> RSLLKTKENLGSGFISLFRGKKIDDDLFEELEEQLLIADVGVETTRKIITNLTEGASRKQLRDAEALYGLLKEEMGEILAKVDEPLNVEGKAPFVILMVGVNGVGKTTTIGKLARQFEQQGKSVMLAAGDTFRAAAVEQLQVWGQRNNIPVIAQHTGADSASVIFDAIQAAKARNIDVLIADTAGRLQNKSHLMEELKKIVRVMKKLDVEAPHEVMLTIDASTGQNAVSQAKLFHEAVGLT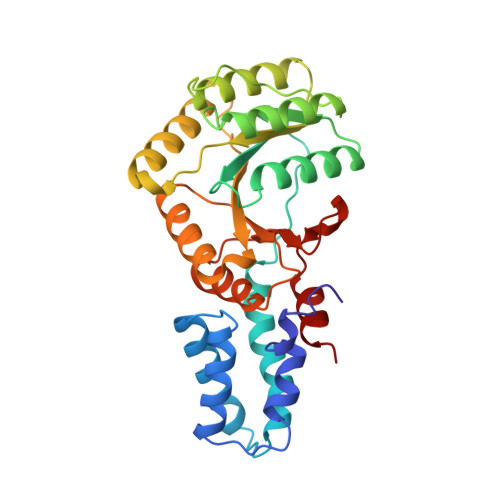GITLTKLDGTAKGGVIFSVADQFGIPIRYIGVGERIEDLRPFKADDFIEALFAR(4S)-4-[(1R)-1-hydroxy-2-({[3-(propan-2-yl)phenyl]methyl}amino)ethyl]-19-(methoxymethyl)-11,16-dioxa-3-azatricyclo[15.3.1.1~6,10~]docosa-1(21),6(22),7,9,17,19-hexaen-2-one 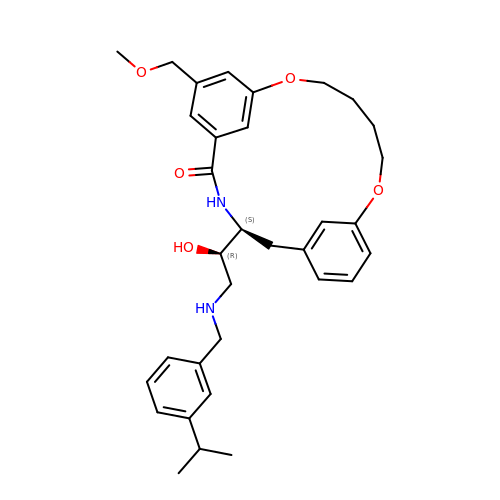| C33 H42 N2 O5 | NGMBHSPURAEOBG-AJQTZOPKSA-N> GAGCAGACGAG;> ACCGCACTCA;> CTGGT;> TCTGAGTGCCGTCTGC

In this work, we exhaustively probe the ability of all 36 immobile HJ sequences to form DNA crystals in two different designed systems. Three separate self-assembling DNA crystal systems are described in this report: the “4 × 5” and “4 × 6” designs (collectively referred to as the 4 × N systems), and a third construct with a “scrambled” sequence variant of the 4 × 6 lattices. Self-assembly was mediated by three constituent oligonucleotides: (S1) containing four sequence repeats of either 5 or 6 bases; (S2) composed of 21 bases containing complementary regions to both (S1); and (S3) which forms the second junction crossover. The HJ serves as the fundamental component at the core of each unit, and the ultimate assembly of the full lattice is facilitated by the complementary 2-base sticky ends that tail each duplex.

The 4 × 5 system robustly crystallized with 75% of the junctions, and we obtained crystals in all but 9 of 36 sequences. In the 4 × 5 system, J25 and J34, both displaying P32 symmetry, crystallized in 50 mM Tris pH = 8.0 buffer containing cobalt hexamine (CoH18N6) and 10 mM MgCl2, and 50 mM HEPES pH = 7.5 with 20 mM MgCl2, respectively. Only cobalt could account for the different peaks in the Fo–Fc maps in J25, whereas in J34, and J22 and J23 in the 4 × 6 and 4 × 6 scramble systems, respectively, contained Mg2+. The modeled ions were readily superimposable, and well-coordinated at Pos1 & 2. Of the resulting structures, 18 exhibited P32 symmetry with average cell dimensions a = b = 68.85 Å c = 60.09 Å, with only nine retaining the original P3221 symmetry with average cell edges a = b = 68.17 Å c = 60.60 Å. Although the cell parameters between the two symmetries were virtually indistinguishable, the differences between the periodicity of the lattices is dramatic, with vastly different cavity sizes. The P32 channels were treated as a hexagonal prism with 6.4 nm along each edge and a height measured from the top to the bottom of each block along with the average c-axis = 6.0 nm, with a resulting volume of ~639 nm3, a nearly 27-fold increase in cavity size relative to the P3221 lattices.>MGDKPIWEQIGSSFIQHYYQLFDNDRTQLGAIYIDASCLTWKGQQFQGKAAIVEKLSSLPFQKIQHSITAQDHQPTPDSCIISMVVGQLKADEDPIMGFHQMFLLKNIND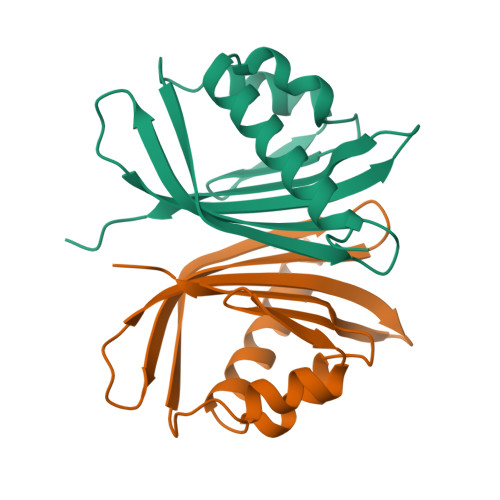AWVCTNDMFRLALHNFG[2x]>[4x]MATNLRG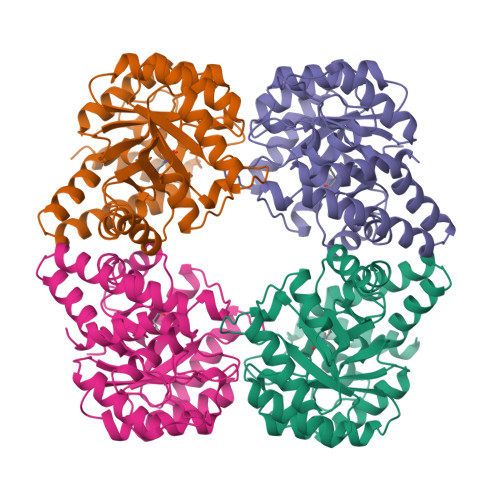VMAALLTPFDQQQALDKASLRRLVQFNIQQGIDGLYVGGSTGEAFVQSLSEREQVLEIVAEEGKGKIKLIAHVGCVTTAESQQLAASAKRYGFDAVSAVTPFYYPFSFEEHCDHYRAIIDSADGLPMVVYNIPALSGVKLTLDQINTLVTLPGVGALKQTSGDLYQMEQIRREHPDLVLYNGYDEIFASGLLAGADGGIGSTYNIMGWRYQGIVKALKEGDIQTAQKLQTECNKVIDLLIKTGVFRGLKTVLHYMDVVSVPLCRKPFGPVDEKYLPELKALAQQLMQERG>PNQSGNWKIIRSENFEELLKVLGVNVMLRKIWVAAASKQAVEIKQEGDTFYIKVSTTVYTTEINFKVGEEFEEQTVDGRPCKSLVKWESENKMVCEQKLLKGEGPKTSWTKELTNDGELILTMTADDVVCTQV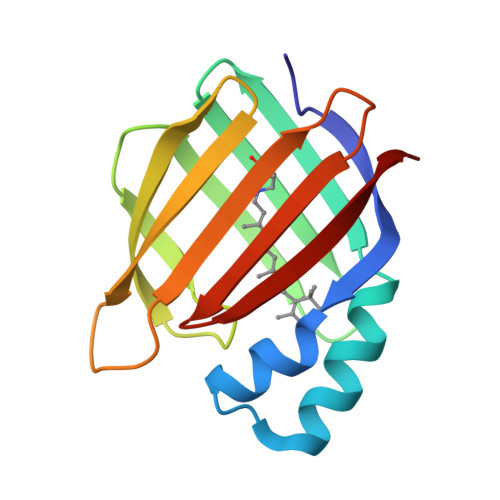FVRE[2x]> SYRPYSYR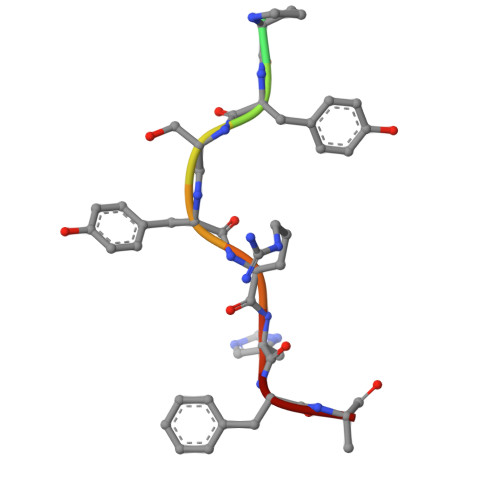HFA> MAQGNNYGQTSNGVADESPNMLVYRKMEDVIARMQDEKNGIPIRTVKSFLSKIPSVFSGSDIVQWLIKNLTIEDPVEALHLGTLMAAHGYFFPISDHVLTLKDDGTFYRFQTPYFWPSNCWEPENTDYAVYLCKRTMQNKARLELADYEAESLARLQRAFARKWEFIFMQAEAQAKVDKKRDKIERKILDSQERAFWDVHRPVPGCVNTTEVDIKKSSRMRNPHKTRKSVYGLQNDIRSHSPTHTPTPETKPPTEDELQQQIKYWQIQLDRHRLKMSKVADSLLSYTEQYVEYDPFLAPPDPSNPWLSDDTTFWELEASKEPSQQRVKRWGFGMDEALKDPVGREQFLKFLESEFSSENLRFWLAVEDLKKRPIREVPSRVQEIWQEFLAPGAPSAINLDSKSYDKTTQNVKEPGRYTFEDAQEHIYKLMKSDSYPRFIRSSAYQELLQAKKKGKSLTSKRLTS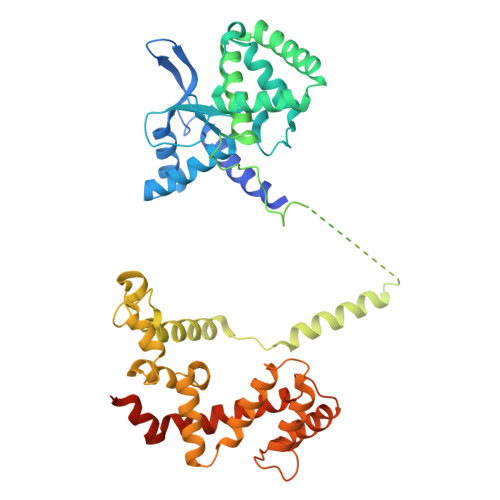LVQSY> NKITPNLAEFAFSLYRQLAHQSNSTNIFFSPVSIATAFAMLSLGTKADTHDEILEGLNFNLTEIPEAQIHEGFQELLRTLNQPDSQLQLTTGNGLFLSEGLKLVDKFLEDVKKLYHSEAFTVNFGDTEEAKKQINDYVEKGTQGKIVDLVKELDRDTVFALVNYIFFKGKWERPFEVKDTEEEDFHVDQVTTVKVPMMKRLG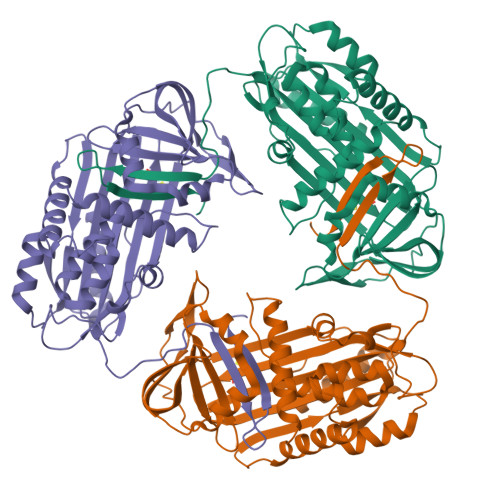MFNIQHSKKLSSWVLLMKYLGNATAIFFLPDEGKLQHLENELTHDIITKFLENEDRRSASLHLPKLCITGTYDLKSVLGQLGITKVFSNGADLSGVTEEAPLKLSKAVHKAVLCIDEKGTEAAGAMFLEAIPRSIPPEVKFNKPFVFLMIEQNTKSPLFMGKVVNPTQK The oxysterol-binding protein (OSBP) and its related proteins (ORP, for OSBP-related protein) have emerged as central regulators of sterol/lipid transport at the junctions formed by ER with other organelles. ORP5 and ORP8 possess the structural features of a lipid transporter: an ER anchor (TMD), a membrane targeting pleckstrin homology (PH) domain and a lipid-binding module (ORD, for OSBP-related domain). Indeed, ORP5 and ORP8, and their yeast counterparts Osh6p and Osh7p, have recently been reported to mediate the counter transport of PtdIns(4)P/phosphatidylserine (PtdSer) between the ER and plasma membrane (PM): ORP5/8 was shown to transfer PtdSer from the ER to PM, coupled with backward transport of PtdIns(4)P from PM to the ER, resulting in its hydrolysis by the phosphatase Sac114–16. Critical to the transport function of ORP5 and ORP8 is their recruitment to the ER–PM MCSs.

To understand the structural principles of ER–PM tethering by ORP5/8, the structure of the ORP8 PH domain was determined by X-ray crystallography. A distinctive feature that stands out, however, is the presence of an unusually long 25 amino acid stretch forming an extended β6–β7 loop (His209–Ser236). Comparative analysis of electrostatic surface of ORP8 PH domain with Osh3p PH domain reveals a distinct positively charged cavity, representing a putative PtdInsP-binding region. The analogous surface on the Osh3p PH domain has a neutral charge suggesting that ORP5 and ORP8 PH domains may possess a distinct PtdInsP-binding mechanism. Close inspection of the distinct positively charged cavity of ORP8 PH domain shows the amino acids forming the basic patch are lined on the β1–β2 and β5–β6 loops (non-canonical mode). Structure-based sequence alignments of related PH domain containing LTPs ORP5, ORP8, OSBP, Cert, and Osh3p establish that the putative PtdInsP residues (red inverted triangles) in ORP5 and ORP8 PH domain are not conserved in OSBP, Cert, and Osh3p. Notably the side chains (green triangles) mediating canonical PtdIns(4)P interaction with OSBP, Cert, and Osh3p are missing in ORP5 and ORP8. To confirm the importance of the non-canonical basic surface for PtdInsP binding, we designed point mutations R136Q, R179Q, and R158Q, R201Q in the ORP5 and ORP8 PH domains, respectively. Both the point mutations in ORP5 and ORP8 PH domains completely abolished the binding to PtdInsPs, confirming that ORP5 and ORP8 PH domain follows a non-canonical PtdInsP-binding regime. While most PH domains (including Osh3, OSBP) utilize the canonical PtdInsP-binding regime for PM targeting, the PH domain of ORP5/8 possesses an atypical PtdInsP-binding site that does not permit PtdIns(4)P binding.

> GSSGIVMADWLKIRGTLKSWTKLWCVLKPGVLLIYKTQKNGQWVGTVLLNACEIIERPSKKDGFCFKLFHPLEQSIWAVKGPKGEAVGSITQPLPSSYLIIRATSESDGRCWMDALELALKSG> IPEYVDWRQKGAVTPVKNQGSCGSCWAFSAVVTIEGIIKIRTGNLNQYSEQELLDCDRRSYGCNGGYPWSALQLVAQYGIHYRNTYPYEGVQRYCRSREKGPYAAKTDGVRQVQPYNEGALLYSIANQPVSVVLEAAGKDFQLYRGGIFVGPCGNKVDHAVAAVGYGPNYILIKNSWGTGWGENGYIRIKRGTGNSYGVCGLYTSSFYPVKN;> MSHNLFTEEDNNKTIRMVIGETFTIELESNPTTGYTWLRSGLAGTELSDCTFAIQSKFNNRAPHDNHKNHRRLLVGAGGTM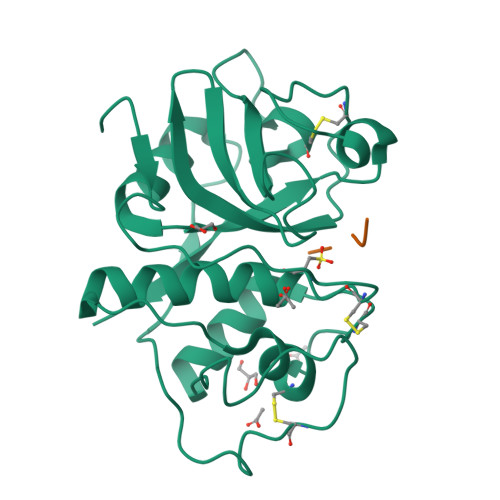VLEVKALKAGKHTLSLAYGRPWVGFNAAAKRYNIHVEATA N-phenylpyrrolidine-1-carboxamide | C11 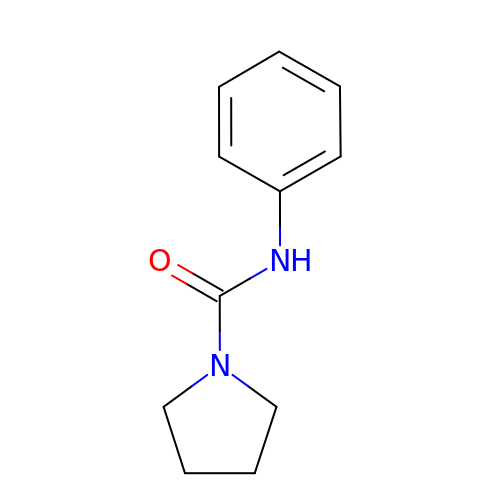H14 N2 O | NTBKXPQLQPBJJL-UHFFFAOYSA-N> RVSIGGTVYTAKK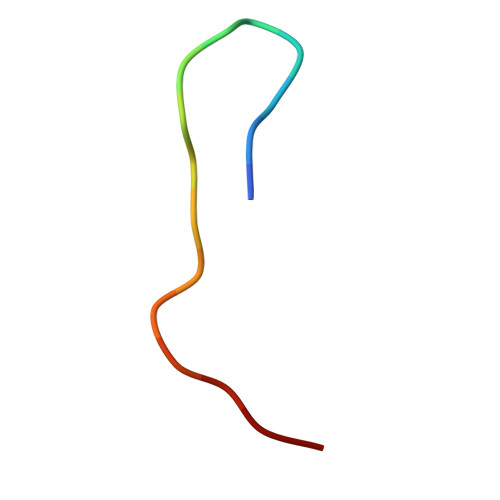YDD>MEISETNIGIFYVSKLLALAPYSAKKNSKGQLEITRSWLFSIYSVCLCLIMVFLTYRGLLFDANSNIPVRMKSATSKVVTASDVSVVVLAIVTGVYCGMFGLRATQELNTRLDKIDSTLSPYNNVKKDRWRAYAMATVSLIVIGILLGLDVGTWVRMAQEMNISDEDTELNVQWYIPFYSLYFILTGLHINFANTAYGLGRRYKRLNQMLRTSYLSADKSYGNATNLVKVSTVKSISFKPMMPMALHASLTKLNTETLPNESATKNKSLLIRAMADNHESLGKCVRLLSRFYGIAVLFILVSCLLHLVATAYFLFLEMLNKRDNGYVWVQMLWIIFHFLRLLMVVEPCHLAAREARKTIQIVCEIERKVFEPILVEETKKFWQQLLVDDAEFSASGLCRVNRTILTSFAS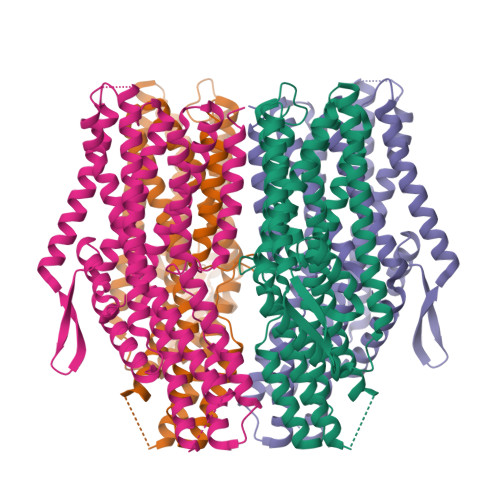AIATYLVILIQFQKTNGLEGGSSGGWSHPQFEK[4x]>[2x]MSQLMGIITRLQSLQETAEAANEPMQRYFEVNG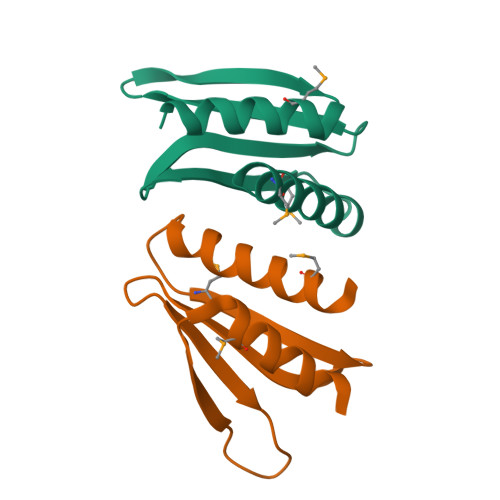EKICSVKYFEKNQTFELTVFQKGEKPNTYPFDNIDMVSIEIFELLQLEHHHHHH> GPKLSLIKVVNGCRLGKIQNLGKAGDCTVDIPGCLLYTRTGSAPHLTHQTLRNIHGVPGIAQLTLSSLAEHHEVLAEYKKGVGSFIGMPESLFYCSLHDPVTPGPAGYVTSKSVSVWGFGGRVEMTVSKFMAIQEALQPDWFQCLSDGEASCAETTSIKRARKSVDRSLLFLDSCLRLQEESEVLQKSVIIGVIEGGDVMEERLRSARETAKRPVGGFLLDGFQGDPAVTETRLHLLSSVTAELPEDKPRLICGVSRPDEVLECIERGVDLFESFFPYQVTERGCALTFTFDCQLNPEETLLQQNGIQEKIKGLDQAKKIEATGCNQEMTSFEINLKEKKYQEDFDPLVRGCSCYCCKNHTRAYIHHLLMTNELLAGVLLMMHNFEHYFGFFCSIREALKND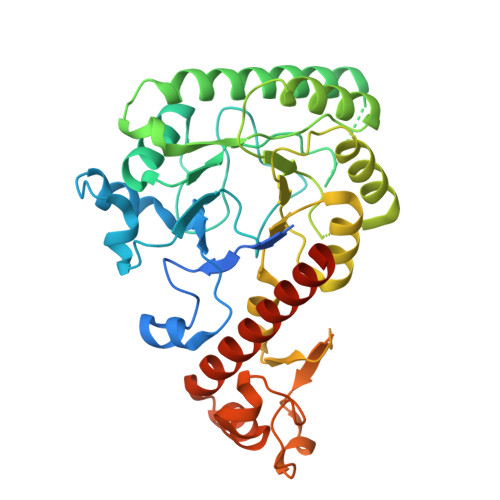TLAQLKELICRQMF> AAPTAYTPLDVAQAYQFP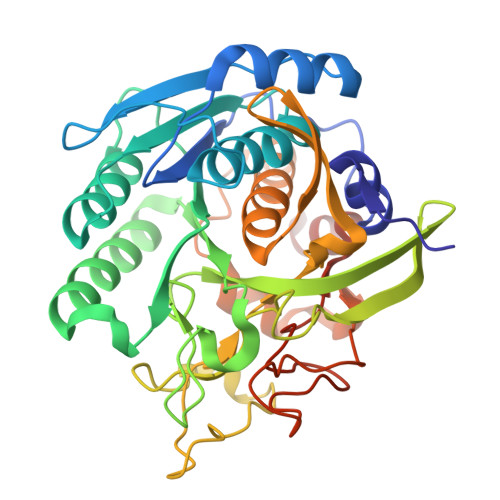EGLDGQGQCIAIIELGGGYDEASLAQYFASLGVPAPQVVSVSVDGASNQPTGDPSGPDGEVELDIEVAGALAPGAKFAVYFAPNTDAGFLDAITTAIHDPTLKPSVVSISWGGPEDSWTSAAIAAMNRAFLDAAALGVTVLAAAGDSGSTDGEQDGLYHVDFPAASPYVLACGGTRLVASGGRIAQETVWNDGPDGGATGGGVSRIFPLPAWQEHANVPPSANPGASSGRGVPDLAGNADPATGYEVVIDGEATVIGGTSAVAPLFAALVARINQKLGKAVGYLNPTLYQLPADVFHDITEGNNDIANRAQIYQAGPGWDPCTGLGSPIGVRLLQALLPSASQPQP> MRLSYEALEWRTPIENSTEPVSLPPPPPFFGQERAREALELAIRGGFHAYLVGPPSLGKHEALLAYLSTQSVETPPDLLYVPLSERKVAVMTLPSGQEIHLAEAVEGLLLEVNRLDELFRQGSFLREKTQLEARFKEAREQQLEALRREAQEAGFALSTNGERLELTGPGPVPAELSARLEEVTLGSLAASAELEVALRRLRRDWALHYLNNRFEPLFQRFPQARAYLEALRARLARYAETGEPLDPAQWRPNLLTSSSSGTPPPIVYEPYATAPRLFGRLDYLVDRGVWSTNVSLIRPGAVHRAQGGYLILDALSLKREGTWEAFKRALRNGQVEPVTEPQAPAGLEVEPFPIQMQVMLVGTPEAFEGLEEDPAFSELFRIRAEFSPTLPASPENCTALGGWLLAQGFQLTQGGLTRLYDEARRMAEQRDRMDARLVEIRALAEEAAVLGGGLLTAESVEQAIAAREHRSFLSEEEFLRAVQEGVIRLRTTGRAVGEVNSLVVVEAAPYWGRPARLTARAAPGRDHLISIDREAGLGGQIFHKAVLTLAGYLRSRYIEHGSLPVTISLAFEQNYVSIEGD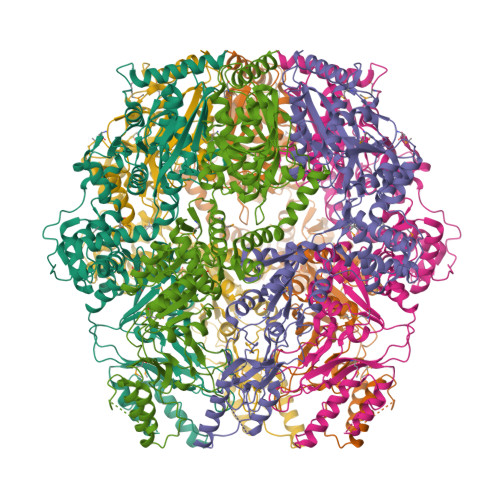SAGLAELVAALSAIGNLPLRQDLAVTGAVDQTGKVLAVGAINAKVEGFFRVCKALGLSGTQGVILPEANLANLTLRAEVLEAVRAGQFHIYAVETAEQALEILAGARMEGFRGLQEKIRAGLEAFARLEEGHDKEDREKLAAALEHHHHHH>[2x]ASLKVTVGTANGKPGDTVTVPVTFADVAKMKNVGTCNFYLGYDASLLEVVSVDAGPIVKNAAVNFSSSASNGTISFLFLDNTITDELITADGVFANIKFKLKSVTAKT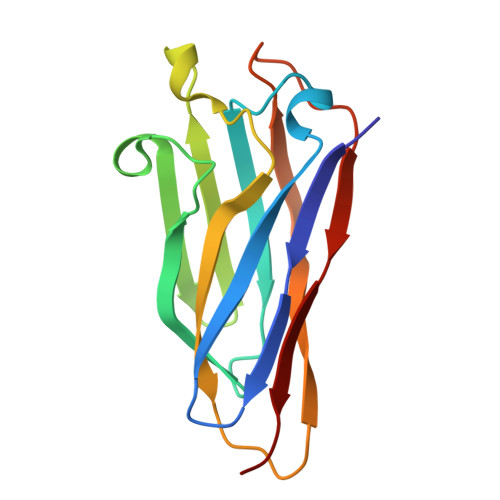TTPVTFKDGGAFGDGTMSKIASVTKTNGSVTIDPG>MNPAAEAEFNILLATDSYKVTHYKQYPPNTSKVYSYFECREKKTENSKLRKVKYEETVFYGLQYILNKYLKGKVVTKEKIQEAKDVYKEHFQDDVFNEKGWNYILEKYDGHLPIEIKAVPEGFVIPRGNVLFTVENTDPECYWLTNWIETILVQSWYPITVATNSREQKKILAKYLLETSGNLDGLEYKLHDFGYRGVSSQETAGIGASAHLVNFKGTDTVAGLALIKKYYGTKDPVPGYSVPAAEHSTITAWGKDHEKDAFEHIVTQFSSVPVSVVSDSYDIYNACEKIWGEDLRHLIVSRSTQAPLIIRPDSGNPLDTVLKVLEILGKKFPVTENSKGYKLLPPYLRVIQGDGVDINTLQEIVEGMKQKMWSIENIAFGSGGGLLQKLTRDLLNCSFK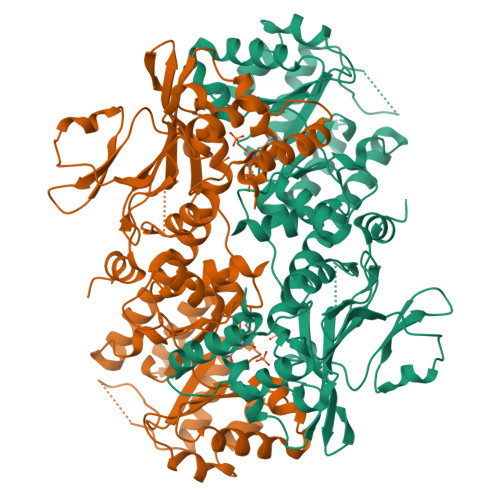CSYVVTNGLGINVFKDPVADPNKRSKKGRLSLHRTPAGNFVTLEEGKGDLEEYGQDLLHTVFKNGKVTKSYSFDEIRKNAQLNIELEAAHH[6x]> XALCDDPRVDRWYCQFV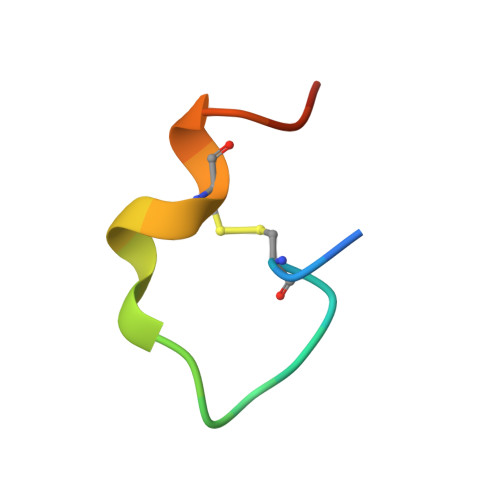EGX11-DEOXY-BETA-RHODOMYCIN 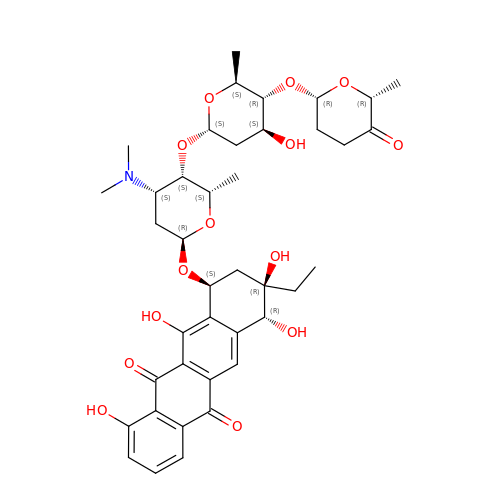| C40 H51 N O14 | OQDCVONZQOVIMP-UNQJTBPASA-N> ERVVIGS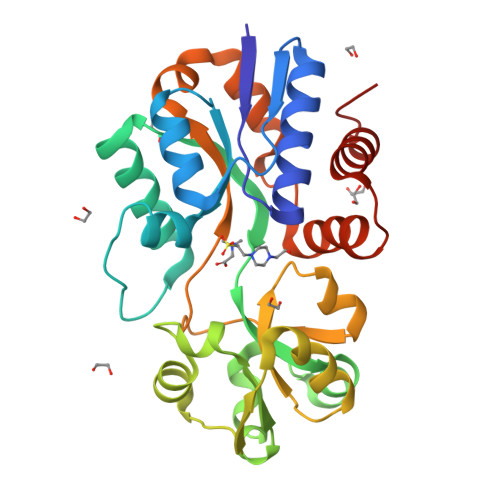KPFNEQYILANMIAILLEENGYKAEVKEGLGGTLVNYEALKRNDIQLYVEYTGTAYNVILRKQPPELWDQQYIFDEVKKGLLEADGVVVAAKLGFRDDAALAVRADWAEENGVEKISDLAEFADQLVFGSDPEFASRPDGLPQIKKVYGFEFKEVKQMEPTLMYEAIKNKQVDVIPAYTTDSRVDLFNLKILEDDKGALPPYDAIIIVNGNTAKDEKLISVLKLLEDRIDTDTMRALNYQYDVEKKDAREIAMSFLKEQGLVK>[2x]GSMAEGGAADLDTQRSDIATLLKTSLRKGDTWYLVDSRWFKQWKKYVGFDSWDKYQMGDQNVYPGPIDNSGLLKDGDAQSLKEHLIDELDYILLPTEGWNKLVSWYTLMEGQEPIARK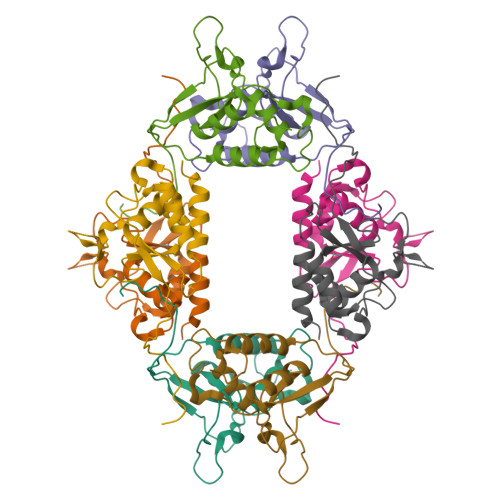VVEQGMFVKHCKVEVYL>[2x]HLVCPMSKSPYVDPHKSGHEIWEEFSMSFTPAVKEVVEFAKRIPGFRDLSQHDQVNLLKAG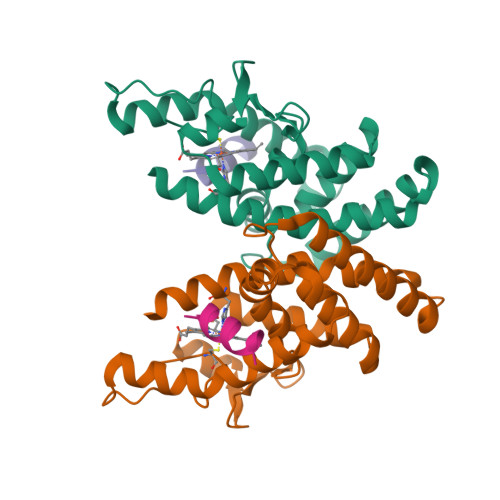TFEVLMVRFASLFDAKERTVTFLSGKKYSVDDLHSMGAGDLLNSMFEFSEKLNALQLSDEEMSLFTAVVLVSADRSGIENVNSVEALQETLIRALRTLIMKNHPNEASIFTKLLLKLPDLRSLNNMHSEELLAFKVHP;>[2x]DPASNLGLEDIIRKALMGSFDDK> MKKICYVLLSLVCVFLFSGCSAGEEASGKKEDVTLRIAWWGGQPRHDYTTKVIELYEKKNPHVHIEAEFANWDDYWKKLAPMSAAGQLPDVIQMDTAYLAQYGKKNQLEDLTPYTKDGTI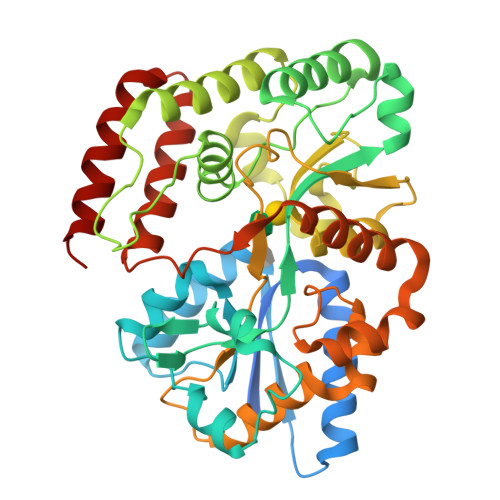DVSSIDENMLSGGKIDNKLYGFTLGVNVLSVIANEDLLKKAGVSINQENWTWEDYEKLAYDLQEKAGVYGSNGMHPPDIFFPYYLRTKGERFYKEDGTGLAYQDDQLFVDYFERQLRLVKAKTSPTPDESAQIKGMEDDFIVKGKSAITWNYSNQYLGFARLTDSPLSLYLPPEQMQEKALTLKPSMLFSIPKSSEHKKEAAKFINFFVNNEEANQLIKGERGVPVSDKVADAIKPKLNEEETNIVEYVETASKNISKADPPEPVGSAEVIKLLKDTSDQILYQKVSPEKAAKTFRKKANEILERNN> MGSSHHHHHHSSGLVPRGSHMASAASYPPIKNTKVGLALSSHPLASEIGQKVLEEGGNAIDAAVAIGFALAVVHPAAGNIGGGGFAVIHLANGENVALDFREKAPLKATKNMFLDKQGNVVPKLSEDGYLAAGVPGTVAGMEAMLKKYGTKKLSQLIDPAIKLAENGYAISQRQAETLKEARERFLKYSSSKKYFFKKGHLDYQEGDLFVQKDLAKTL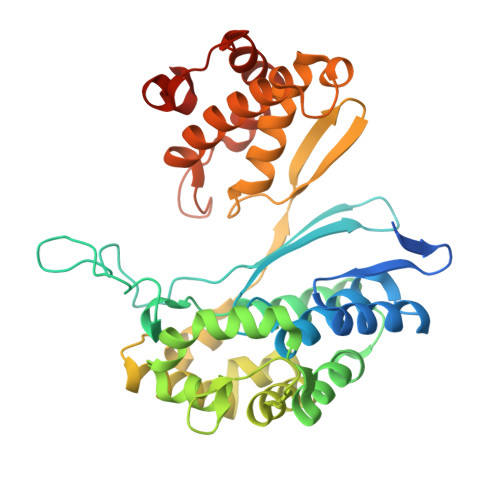NQIKTLGAKGFYQGQVAELIEKDMKKNGGIITKEDLASYNVKWRKPVVGSYRGYKIISMSPPSSGGTHLIQILNVMENADLSALGYGASKNIHIAAEAMRQAYADRSVYMGDADFVSVPVDKLINKAYAKKIFDTIQPDTVTPSSQIKPGMGQLHEGSN> GMFKPQGLYDYICQQWQEEILPSLCDYIKIPNKSPHFDAKWEEHGYMEQA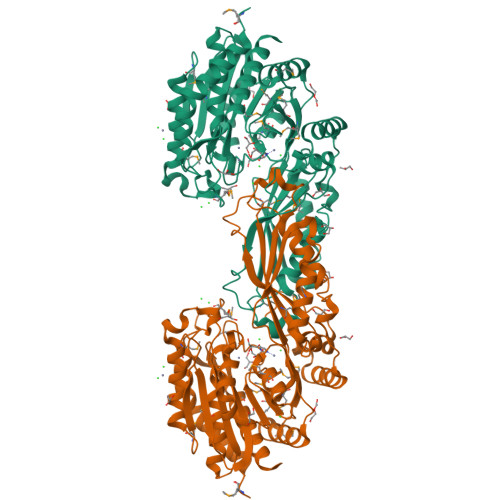VNHIANWCKSHAPKGMTLEIVRLKNRTPLLFMEIPGQIDDTVLLYGHLDKQPEMSGWSDDLHPWKPVLKNGLLYGRGGADDGYSAYASLTAIRALEQQGLPYPRCILIIEACEESGSYDLPFYIELLKERIGKPSLVICLDSGAGNYEQLWMTTSLRGNLVGKLTVELINEGVHSGSASGIVADSFRVARQLISRIEDENTGEIKLPQLYCDIPDERIKQAKQCAEILGEQVYSEFPWIDSAKPVIQDKQQLILNRTWRPALTVTGADGFPAIADAGNVMRPVTSLKLSMRLPPLVDPEAASVAMEKALTQNPPYNAKVDFKIQNGGSKGWNAPLLSDWLAKAASEASMTYYDKPAAYMGEGGTIPFMSMLGEQFPKAQFMITGVLGPHSNAHGPNEFLHLDMVKKLTSCVSYVLYSFSQKK>[2x]MSIVVKNNIHWVGQRDWEVRDFHGTEYKTLRGSSYNSYLIREEKNVLIDTVKHKFSREFVQNLRNEIDLADIDYIVINHAEEDHAGALTELMAQIPDTPIYCTANAIDSINGHHHHPE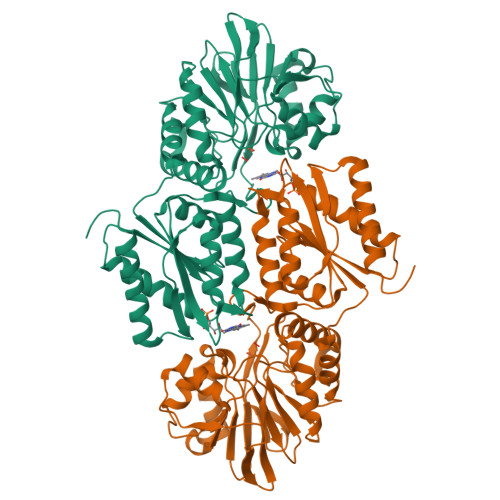WNFNVVKTGDTLDIGNGKQLIFVETPMLHWPDSMMTYLTGDAVLFSNDAFGQHYCDEHLFNDEVDQTELFEQCQRYYANILTPFSRLVTPKITEILGFNLPVDMIATSHGVVWRDNPTQIVELYLKWAADYQEDRITIFYDTMSNNTRMMADAIAQGIAETDPRVAVKIFNVARSDKNEILTNVFRSKGVLVGTSTMNNVMMPKIAGLVEEMTGLRFRNKRASAFGSHGWSGGAVDRLSTRLQDAGFEMSLSLKAKWRPDQDALKLCREHGREIARQWALAPLPQSTVNTVVKEETSATTTADLGPRMQCSVCQWIYDPAKGEPMQDVAPGTPWSEVPDNFLCPECSLGKDVFEELASEAK>[4x]MNPAAEAEFNILLATDSYKVTHYKQYPPNTSKVYSYFECREKKTENSKLRKVKYEETVFYGLQYILNKYLKGKVVTKEKIQEAKDVYKEHFQDDVFNEKGWNYILEKYDGHLPIEIKAVPEGFVIPRGNVLFTVENTDPECYWLTNWIETILVQSWYPITVATNSREQKKILAKYLLETSGNLDGLEYKLHDFGYRGVSSQETAGIGASAHLVNFKGTDTVAGLALIKKYYGTKDPVPGYSVPAAEHSTITAWGKDHEKDAFEHIVTQFSSVPVSVVSDSYDIYNACEKIWGEDLRHLIVSRSTQAPLIIRPDSGNPLDTVLKVLEILGKKFPVTENSKGYKLLPPYLRVIQGDGVDINTLQEIVEGMKQKMWSIENIAFGSGGGLLQKLTRDLLNCSFKCSYVVTNGLGINVFKDPVADPNKRSKKGRLSLHRTPAGNFVTLEEGKGDLEEYGQDLLHTVFKNGKVTKSYSFDEIRKNAQLNIELEAAHH

Nicotinamide phosphoribosyltransferase (NAMPT) is the rate-limiting enzyme of the NAD+ salvage pathway, having an SL relationship with nicotinic acid phosphoribosyltransferase (NAPRT), the key enzyme in the NAD+ Preiss-Handler pathway. NAMPT exists as a homodimer in solution 29, 30. Monomeric NAMPT has a modular structure consisting of two domains. Two monomers are arranged to form a dimer in a head-to-tail manner, where the first domain of one monomer is assembled with the second domain of the other monomer to form the active site, indicating the presence of two active sites in the dimer.

To determine whether A4276 inhibits NAMPT through direct binding, and to elucidate its mechanism of action, we solved the crystal structure of the NAMPT-A4276 complex which showed clear electron densities for A4276. The asymmetric unit of the crystal structure contains two dimers of the complex, with dimer-1 composed of molecules A and B, and dimer-2 composed of molecules C and D. The crystal structures of dimer-1 and dimer-2 were superimposed with a root-mean-square deviation of 0.204 Å for all equivalent Cα atoms. A4276 nestles in the U-shaped central β-sheet of the second domain, adopting a V-shaped conformation with a kink at the C10 atom. The structure of A4276 comprises three parts: nicotinamide, benzene, and 6-methylbenzoxazole groups. The active site of NAMPT can be divided into subsites-I, -II, and -III, which accommodate nicotinamide, benzene, and 6-methylbenzoxazole, respectively. Through extensive π-π stacking interactions, the pyridine ring of nicotinamide is trapped between Tyr18 and Phe193 of subsite-I, where the substrate nicotinamide ring binds. The amide group of A4276 makes polar interactions with Asp219 and a water molecule in subsite-I; the -NH group is hydrogen-bonded to the side-chain carboxylate of Asp219, and the carbonyl oxygen is connected to a water molecule interacting with Ser275 and Ala245. The benzene ring of A4276 is nestled in the hydrophobic subsite-II lined by His191, Val242, Ile351, and the Cβ atom of Ser275. In contrast, only one side of 6-methylbenzoxazole interacts with Ala379, Ile309, and the hydrophobic part of the side chain of Arg349 in subsite-III, while the other side is exposed to the solvent. Overall, the crystal structure revealed that A4276 binds to the active site of NAMPT exclusively through non-covalent interactions.Here we report seven high-resolution cryo-EM structures of filamentous peptide nanotubes based on a cross-α supramolecular architecture that provide insight into the designability of helical peptide filaments. A structural interaction is identified based on an appropriately placed pair of arginine residues (RxxxR) within the corresponding peptide sequences. This local interaction motif, designated as an arginine clasp, is robust within the context of these cross-α assemblies and can guide the coalescence of helical protofilaments into structurally defined cross-α nanotubes. In contrast to most structurally characterized filaments based on synthetic α-helical coiled-coils, the chain axes of the helical protomers are oriented in a plane nearly perpendicular to the long axis of the assembly.

Each nanotube was derived from coalesence of three protofilaments derived from the dimeric protomer. Among all three structures, the helices within the dimeric asymmetric unit could be superimposed with only minimal differences. Structural overlays of laterally interacting protofilaments indicated a conservation of the interfaces between the three filament structures. However, the axial interactions along the contour length of a protofilament for the Form II-like assemblies appeared quite robust and comparable in energy and buried surface area to that of Form I protofilaments.

>[104x]QAEILKADAEILKAYAKILEAHAEILKAQ>[3x]SDGGKVVAATTAQIQEFTKYAGIAATAYCRSVVPGNKWDCVQCQKWVPDGKIITTFTSLLSDTNGYVLRSDKQKTIYLVFRGTNSFRSAITDIVFNFSDYKPVKGAKVHAGFLSSYEQVVNDYFPVVQEQLTAHPTYKVIVTGHSLGGAQAL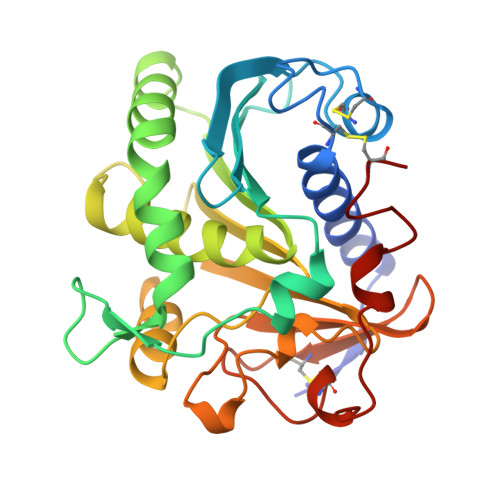LAGMDLYQREPRLSPKNLSIFTVGGPRVGNPTFAYYVESTGIPFQRTVHKRDIVPHVPPQSFGFLHPGVESWIKSGTSNVQICTSEIETKDCSNSIVPFTSILDHLSYFDINEGSCL Non-ribosomal peptide synthetases are important enzymes for the assembly of complex peptide natural products. Within these multi-modular assembly lines, condensation domains perform the central function of chain assembly, typically by forming a peptide bond between two peptidyl carrier protein (PCP)-bound substrates. To address this, we report the structure and biochemical characterization of complexes of a PCP domain bearing a stable analog of the acyl acceptor complexed to the acceptor site of a C domain from the NRPS that biosynthesizes fuscachelin in the thermophile Thermobifida fusca. The C3 domain of the didomain resembles other members of its class, comprising a pseudo-dimer of CAT domains with bridge (R2923 to T2944) and floor loop (A2843 to L2858) regions.

To verify the role of the R2577 in controlling access to the catalytic channel, we generated the Arg to Gly mutant (R2577G) of the C3 domain. To control the modification state of the PCP2 domain, the mutant PCP2-C3 didomain construct was expressed in the entD mutant of E. coli. Similar to the wild-type construct, the protein expressed well and crystallized in the same conditions. The structure of the R2577G mutant is very similar to that of the wild-type protein, with the PCP2 domain sitting at the acceptor site of the C3 domain (RMSD (all atoms) 1.2 Å compared to wild type). The first noticeable difference is a small rotation of the PCP domain in relation to the C domain and slight alterations in the PCP interacting regions of the C domain, likely attributable to the R2577G mutation allowing the first helix of the C domain to sit deeper in the acceptor channel. The major difference, however, is the positioning of the PPant moiety, which now fully extends thought the acceptor channel into the active site in a similar way to that seen in the ObiF1, SrfA-C, and AB3403 structures. This observation supports the hypothesis that R2577 acts to control substrate access to the active site of the C domain. Firstly, we confirmed that the R2577G mutant C domain retained activity (with Gly), although this was reduced compared to the wild-type C domain (32%), possibly due to the loss of stabilizing interactions with the PPant arm. Whilst this residue is largely conserved in LCL domains, it is typically Gly or other small residues in DCL domains, which we have confirmed allows the unmodified PPant into the C-domain active site.

>VTAYEEIVCQVFAAVLDRSDVTADADFFALGGHSLLSLRVVARLRALLGVDVGVRDLFEAPTPAALAARLTTQTGRRPAVTRRGPDAPPVLSHFQRGLWLIEQVYQTRGAYNVPLAVHVSDRLDLDVLRAAVRDLVARHEVLRTLVRSSDDGPDPVLLAPEDAAVDVAEVQAAGPVADLLAELTAQPFDLATQIPLRVRMITGEQVDGCVLLLVCHHIAADEWSFAPLLRDLDTAYRARAAGRAPDWEPLPAQYSDYAATLHDWLGEATDPASPLRRQLDYWQHALQDLPDELDLPTDRPRPATASHRGGLARAELPPELVEAVRRLAAQHGVTVFMVVQAAVAVLLHRLGAGDDIPLGSPVADRADEAVHDTVGFFLNTLVLRVNLSGNPTFADLLDRVRAVDLEAFARADAPFDAVVDTVKPPRAVSRHPLFQTMVSYQRRPSDVDRLFGAATRLVEVPLDTAKFDLEFAFIEDGHGGAHIALNYAADLFDHDSAEQLVARLRTVLEHACADPCRPVAGVEVVSGA[2x]>KKYFMSSVRRMPLNRAKALCSELQGTVATPRNAEENRAIQNVAKDVAFLGITDQRTENVFEDLTGNRVRYTNWNEGEPNNVGSGENCVVLLTNGKWNDVPCSDSFLVVCEFS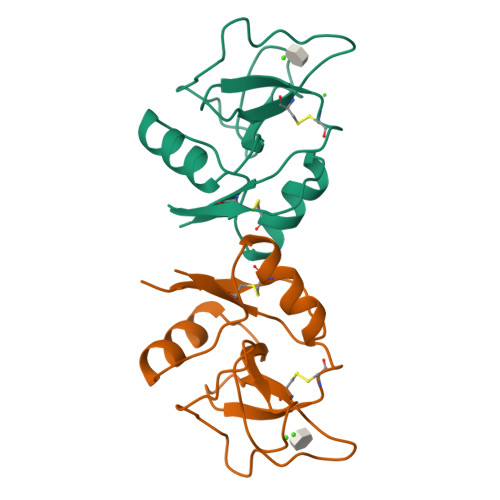D[2x]> MAIDFLVNILELIKEKQCNINLFSAISLTSIVYNNFGEFLSNNQSYSTNNPLLKYHIIILNDKNKTKDVEEKRNIFKREVAELISRNFKLDGEKVRNYFDSLKEVLKSLKYTIVDVEITTRTRALIGVSTSLGKLIFGSGISFDPYMNLPYIPASEIKGIVRSYIEGKLGEQEAEEIFGNEEREGNVNFTDAYPTRSKDFLFVPDVITPHYNGKKSEADAEPRPVIHLTIAPKVTFRFLIYYKREDVGKPICDSMPIILIRGLGARSSVGYSLFELRKIEVIKAAAHHHHHHH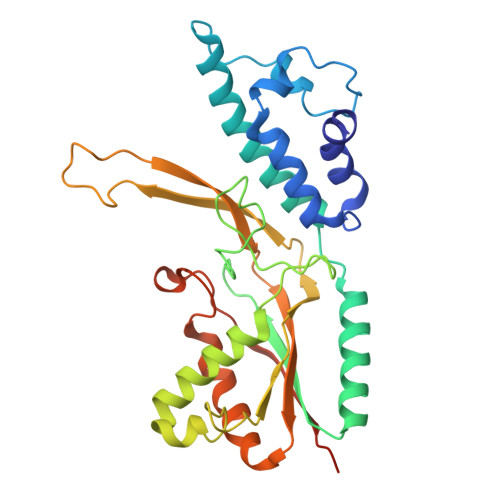HHH>[2x]SNAANIQLVNGKGMAQAAAQSRTTTVTLKARRGKIMDTNGAILAQSVERYTIIGNPEQA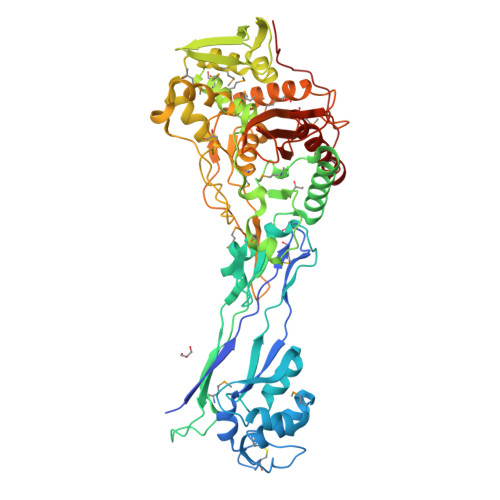QAFIPTTCTKQTGSNCHQINGKPVGVTGAAAVARLLAPVLGMDATELGAKLSISGQYVVLKKDVTPAVKRKISKLNLGGIVYAELSNERLYSNGTLMGSLLGGVDADGKGVAGIEQMENKTLTGRDGYQVYQQGNSGVEIPGTMTESKDAVNGSDVTLTIDRDVQWYTEKVLSDSENKYHSAWGIAMVQDVQSGDILALADSDTTEAGSDQAKMGASRAVSETFEPGSIGKVLAMSGMLQLGLHKIDDKFTVPNTVTVEGQTYKDAVDHGNEHWTLAGILEQSSNVGMVIAGDKMTNEQRYNFISKFGIGQATGLNLPGESEGVLHPSDSWDRRTRNTVLFGQGYTVNVMQLTNAISVIANKGVKKPQRIIKSITDTAGHVEEQQSKGEATRVIDESVASQMLNAMESSAEHYNTFVKVDGYRMAAKSGTAEVAGANGQLTSIISDYSTIIPADNPRFVITVVLKDPQGSFGGLTAGPVTAEIGEFLMQKYEVPASSPRTDAIPVNW>AKLETVTLGNIGKDGKQTLVLNPRGVNPTNGVASLSQKGCVPALEKRVTVSVSQPSRNRKNYKVQVKIQNPTACTANGSCDPSVTRQAYADVTFSFTQYSTCEERAFVRTELAALLASPLL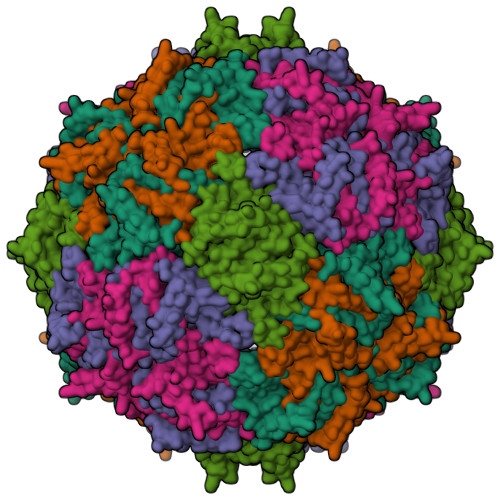IDAIDQLNPAY[5x]> MGPSSGSRLGPPEAESPSQPPKRRKKRYLRHDKPPYTYLAMIALVIQAAPSRRLKLAQIIR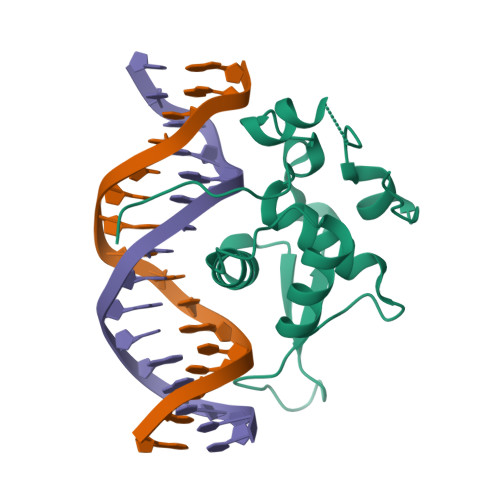QVQAVFPFFREDYEGWKDSIRHNLSSNRCFRKVPKDPAKPQAKGNFWAVDVSLIPAEALRLQNTALCRRWQNGGARGAFAKDLGPYVLHGRPYRPPSPPPPPSEGFSIKSLLGGSGEGAPWPGL> GGADPKKVLDQAKDQMENVVRTLKQELEE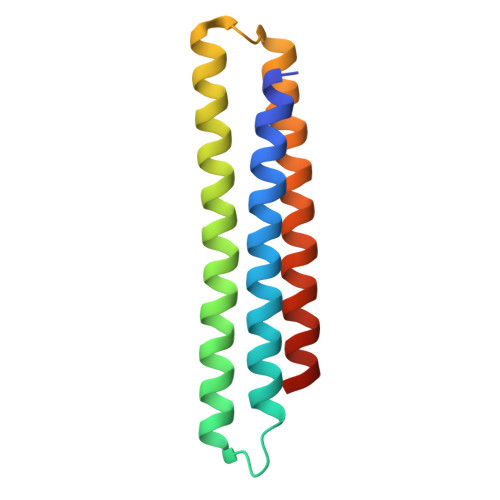LAKEARKLDLTQSEKIELKLRYIVAHLAAIGDIEEAIREAKEEADKLKRAGLVNSQQFDEFKRRLEELHKEADRKRADYAEEFRNKLEYG>GGSVKLEMEMVTQQYEKAKAIQDEQLERLTQICQEQGFEIRQLRAHLAQQDLDLAAEREAALQ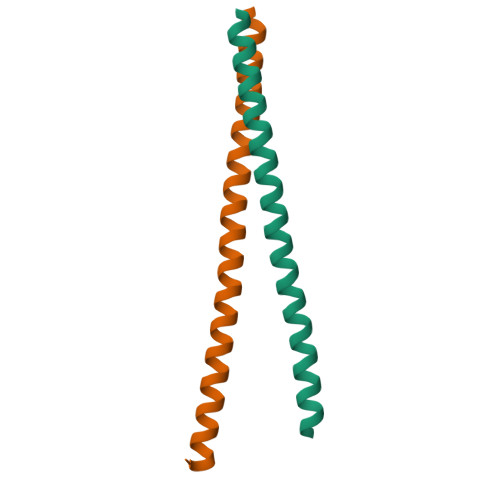A[4x]> DAASHEERMNNYRKRVGRLFMEQKAAQPDAVKLPSGLVFQRIARGSGKRAPAIDDKCE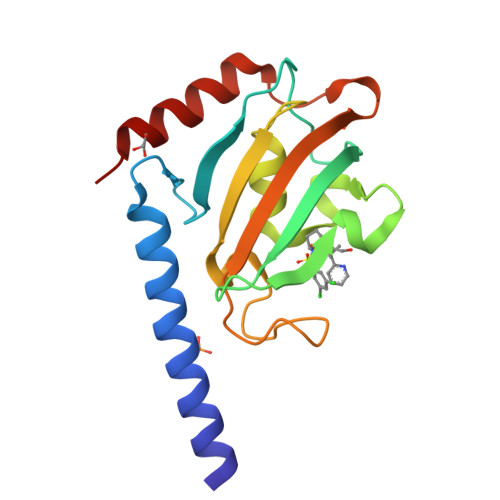VHYTGRLRDGTVFDSSRERGKPTTFRPNEVIKGWTEALQLMREGDRWRLFIPYDLAYGVTGGGGMIPPYSPLEFDVELISIKDGGKGRTAEEVDEILRKAEEDRE> AQKPVDNITQIIGGTPVVKLRNVVDDNAADVYVKLEYQNPGGSVKDRIALAM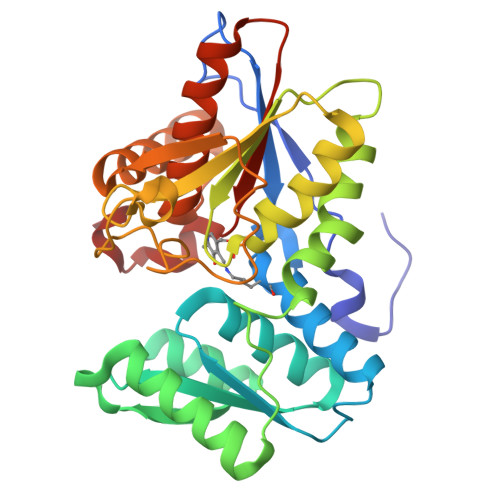IEKAEREGKIKPGDTIVEPTSGNTGIGLAFVCAAKGYKAVFTMPETMSQERRNLLKAYGAELVLTPGSEAMKGAIKKAKELKEEHGYFEPQQFENPANPEVHELTTGPELLQQFEGKTIDAFLAGVGTGGTLSGVGKVLKKEYPNIEIVAIEPEASPVLSGGEPGPHKLQGLGAGFIPGTLNTEIYDSIIKVGNDTAMEMSRRVAKEEGILAGISSGAAIYAAIQKAKELGKGKTVVTVLPSNGERYLSTPLYS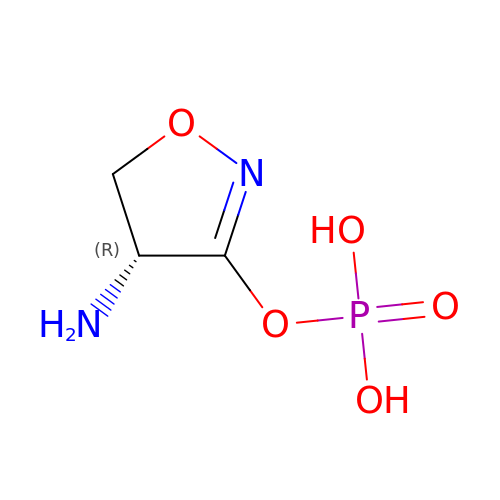[(4R)-4-azanyl-4,5-dihydro-1,2-oxazol-3-yl] dihydrogen phosphate | C3 H7 N2 O5 P | SFMNESRSKJTEMJ-UWTATZPHSA-N>MAKVSLEKDKIKFLLVEGVHQKALESLRAAGYTNIEFHKGALDDEQLKESIRDAHFIGLRSRTHLTEDVINAAEKLVAIGAFAIGTNQVDLDAAAKRGIPVFNAPFSNTRSVAELVIGELLLLLRGVPEANAKAHRGVWNKLAAGSFEARGKKLGIIGYGHIGTQLGILAESLGMYVYFYDIENKLPLGNATQVQHLSDLLNMSDVVSLHVPENPSTKNMMGAKEISLMKPGSLLINASRGTVVDIPALADALASKHLAGAAIDVFPTEPATNSDPFTSPLAEFDNVLLTPHIGGSTQEAQENIGLEVAGKLIKYSDNGSTLSAVNFPEVSLPLHVV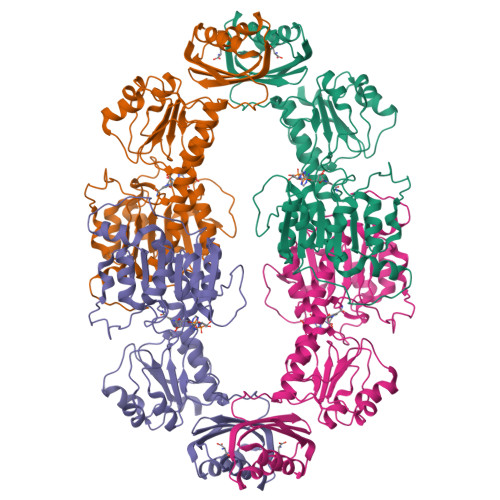RRLMHIHENRPGVLTALNKIFAEQGVNIAAQYLQTSAQMGYVVIDIEADEDVAEKALQAMKAIPGTIRARLLY[2x]> GSHMASGEGPALYEDPPDQKTSPSGKPATLKICSWNVDGLRAWIKKKGLDWVKEEAPDILCLQETKCSENKLPAELQELPGLSHQYWSAPSDKEGYSGVGLLSRQCPLKVSYGIGDEEHDQEGRVIVAEFDSFVLVTAYVPNAGRGLVRLEYRQRWDEAFRKFLKGLASRKPLVLCGDLNVAHEEIDLRNPKGNKKNAGFTPQERQGFGELLQAVPLADSFRHLYPNTPYAYTFWTYMMNARSKNVGWRLDYFLLSHSLLPALCDSKIRSKALGSDHCPITLYLAL

Mammalian AP endonuclease 1 (APE1) initiates repair of abasic (apurinic/apyrimidinic) sites and other toxic and mutagenic DNA lesions and performs critical roles in base excision repair (BER) and single strand break repair (SSBR). APE1 hydrolytically cleaves phosphodiester bonds at abasic sites, which arise through spontaneous rupture of the N-glycosyl bond (depurination) or by the activity of DNA glycosylases, which initiate BER. APE1 is the major mammalian enzyme for repair of abasic sites, which impair DNA replication and other processes, causing DNA strand breaks and cross links. In addition to its AP endonuclease activity, the exonuclease activity of APE1 processes BER intermediates generated by bifunctional DNA glycosylases and removes 3´-blocking groups arising at strand breaks.

S6 Fig New structure of apo human APE1 with a focus on the remote binding pocket. For this model the resolution cutoff was 1.25 Å. (b) The same view of a model that was refined using the same diffraction data but with a resolution cutoff of 1.40 Å. The figure shows no significant change in electron density relative to that observed for the model refined with a resolution cutoff of 1.25 Å. Superposition of the structures for these apo forms of human APE1 (wild-type and C138A) indicates that the overall conformations are very similar, with RMSD values of 0.100 Å for backbone Cα atoms and 0.247 Å for all non-hydrogen atoms, with minor structural differences in the remote binding pocket near C138. A superposition of our new structure for apo-APE1 and a prior structure of Mg2+-bound APE1 illustrates that binding of Mg2+ causes substantial conformational changes in APE1, most near the Mg2+ site, as expected. The Mg2+-induced NMR shift perturbations reflect these conformational changes, in addition to changes in the chemical environment near the Mg2+-binding site. Regarding APE1 conformational changes caused by the binding of compound 3, superposition of our two new structures for apo APE1, free and in complex with compound 3, reveals that binding of 3 induces minor changes in overall structure with some significant changes in the remote binding site for residues including L62, D90, R136, Q137, F162, S164, F165, and L318.>[3x]SDKI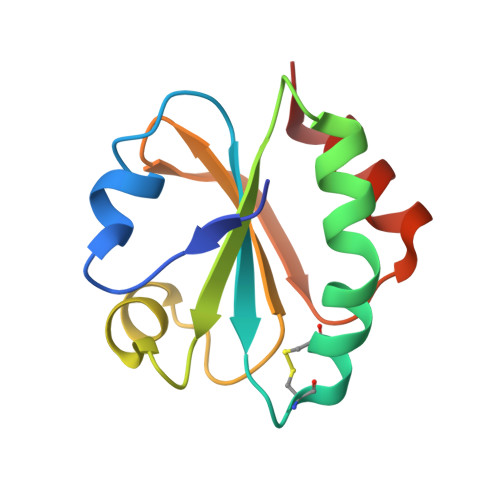IHLTDDSFDTDVLKADGAILVDFWAEWCGACKMIAAILDEIADEYQGKLTVAKLNIDQNAGTAAKYGIRGIATLLLFKNGEVAATKVGALSKGQLKEFLDANLA>[2x]NAMQDIHFRRHYVRHLPKEVSQNDI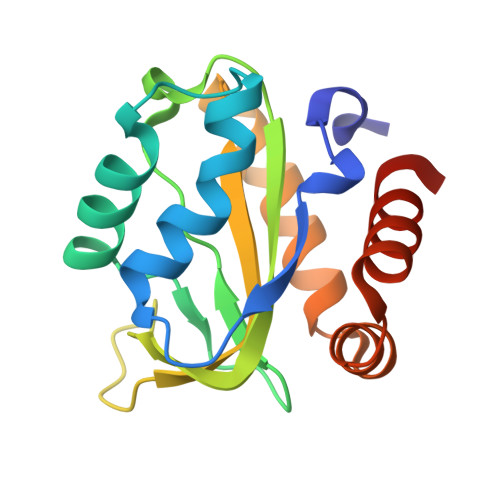IKALASPLINDGMVVSDFADHVITREQNFPTGLPVEPVGVAIPHTDHKYVRQNAISVGILAEPVNFEDMGGEPDPVPVRVVFMLALGESNKQLNVLGWIMDVIQDEDFMQQLLVMNDDEIYQSIYTRISERGEV>[6x]MDRMKIEAVIFDWAGTTVDYGCFAPLEVFMEIFHKRGVAITAEEARKPMPLLKIDHVRALTEMPRIASEWNRVFRQLPTEADIQEMYEEFEEILFAILPRYASPINAVKEVIASLRERGIKIGSTTGYTREMMDIVAKEAALQGYKPDFLVTPDDVPAGRPYPWMCYKNAMELGVYPMNHMIKVGDTVSDMKEGRNAGMWTVGVILGSSELGLTEEEVENMDSVELREKIEVVRN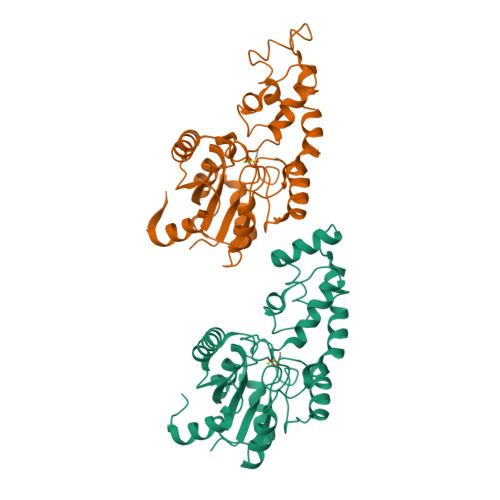RFVENGAHFTIETMQELESVMEHIEKQELIIS2-O-methyl-alpha-D-galactopyranose | C7 H14 O6 | 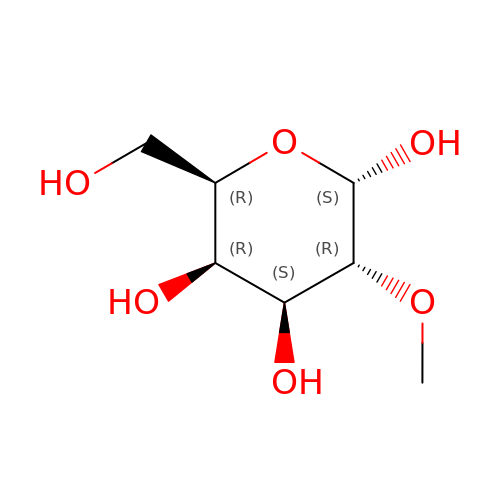UMPNFVHHMOSNAC-PZRMXXKTSA-N The subject of this study, the JC virus (JCV), is a member of this family and the causative agent of a brain disease termed Progressive Multifocal Leukoencephalopathy (PML), a disease that is often fatal and for which there is no cure. Herein we present the high-resolution crystal structure of the origin binding domain (OBD) from the JCV initiator protein large T-antigen. The T-antigens encoded by polyomaviruses are multi-domain, multifunctional proteins that form hexamers and double hexamers at origins of replication. The topology of the JCV OBD is a five-stranded antiparallel β-sheet sandwiched between two helices on either side.

The JCV OBD (residues 132–261) crystallized in three different forms that were termed form 1, form 2 and form 3. Form 1 has two molecules in the asymmetric unit cell, and together the three crystals provide four independent structures of the JCV OBD. JCV OBD region B3 (residues 216–220) is poorly ordered in crystal forms 1 and 2, but well ordered in form 3. Crystal form I crystallized with two OBDs in the asymmetric unit. The molecules are orientated in a head-to-tail manner and situated at approximately right angles to each other (94.5°). This dimer contains a small interface (∼550 Å2) that is buried between the adjacent JCV OBDs. Therefore, we examined the higher order structure that the JCV T-ag OBD adopts in crystal form 1. Interestingly, the JCV OBD forms a right-handed tetrameric spiral. The angle between the monomers is ∼900 and the rise per monomer is ∼9 Å.

>[2x]GSKVEDPKDFPVDLHAFLSQAVFSNRTVASFAVYTTKEKAQILYKKLMEKYSVTFISRHGFGGHNILFFLTPHRHRVSAINNYCQKLCTFSFLICKGVNKEYLFYSALCRQPYAVVEESIQGGLKEHDFNPE> MAGALRLVLGDQLSDNLSALVDADLSRDQVLMVESRVEATAWKHHKQKLVLVWSAMRQFAERLRARGFNVRYVTLEDPDNTGSIGGELRRALEARAFDRVIRTACGKWGLESHLLSLDLPVPMETREDDRFLCSRAQFAAWAEGRRELRMEFFYREMRRKTGLLMDGDQPAGGRWNFDAENRRKLPPGLRPPERLRIPPNPTTQTVLEQVSRGFDDHFGEVEGFGWPTNPDEATAILDHFIADMLPSFGDWQDAMSWRRPFLWHSLISPALNIGLLDPLDICRRAEAAWREGRAPLNAVEGFIRQIIGWREFVRGIYWLKMPEYAQRNALDAQGKLPGFYWTGQTDMACVADTVRAAHDHAYAHHIQRLMVTGNLAMLLGVHPDAVDDWYMVVFADAYEWVEMPNTRGMATFADGGIVGSKPYAASGAYIDRMSDYCKGCRYDVKKRLGDDACPFNALYWDFIDRHAQRLAGNGRMMMPLRTLEKMPDAEREAFRKQARALRVKMGVSG

Photolyases repair UV damage to DNA by using absorbed blue light. Within the photolyase/cryptochrome superfamily (PCSf), a major subgroup consists of prokaryotic (6–4) photolyases. These enzymes rely on flavin adenine dinucleotide (FAD) as a catalytic cofactor, besides an ancillary antenna chromophore, and a [4Fe-4S] cluster with yet unknown function. For the prokaryotic 6–4 photolyase of Caulobacter crescentus, we investigated structural changes associated with its different redox states by damage-free crystallography using X-ray free-electron lasers.

In the oxidized state of Cc(6–4)PL, the [4Fe-4S] cluster adopts its characteristic rhomboid geometry, which is identical in the synchrotron and XFEL structures. Notably, in the synchrotron-derived Cc(6–4)PL structures of the FADox state, Wat1 is displaced into the same direction, albeit by only <0.5 Å. This may be a consequence of partial FAD reduction due to radiation damage by synchrotron X-ray irradiation as observed before in class I and II PLs.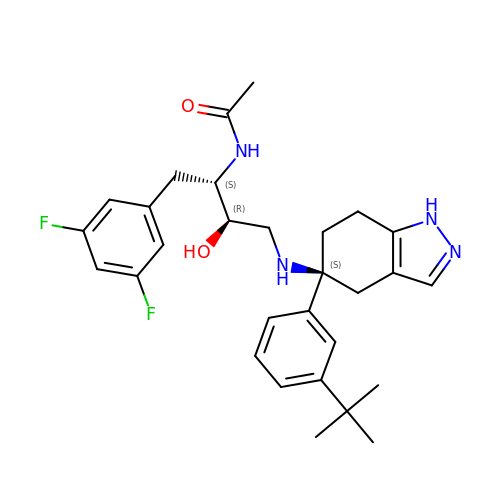N-[(1S,2R)-3-{[(5S)-5-(3-tert-butylphenyl)-4,5,6,7-tetrahydro-1H-indazol-5-yl]amino}-1-(3,5-difluorobenzyl)-2-hydroxypropyl]acetamide | C29 H36 F2 N4 O2 | BAILJXDQIBWAPX-GKRYNVPLSA-N> STGVKFQVGDLVWSKVGTYPWWPCMVSSDPQLEVHTKINTRGAREYHVQFFSNQPERAWVHEKRVREYK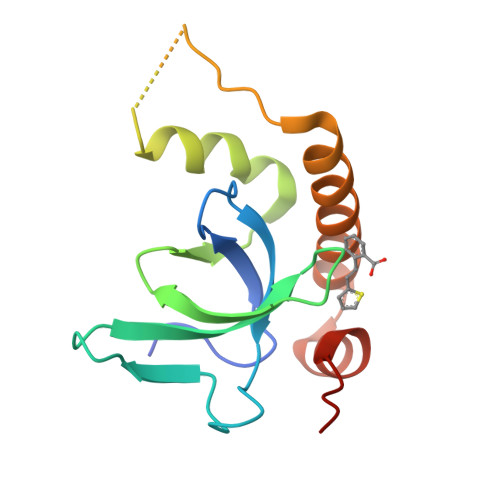GHKQYEELLAEATKQASNHSEKQKIRKPRPQRERAQWDIGIAHAEKALKMTREERIEQYTFIYIDKQ>MGRENVLPVHNDVYEDFVFTTPYFQPESTFKSVPKLFSDILLGGVEWVYTTSESVLAYDYKLWYLWSGVSNLDESFDMFFNQYWALSLSTSVFQLFYAVILDRYLSVLFQNTPYTNDWFRMMLHSKETALIWLYHPELSWHINGLNQFFTYFYGGILEFVYFDKSNPDMCILVHTLWIHLLILFLIFTGFVTILFSFYGNPNTEENTIDSDYLAASGTVEAEKEITSIDDYLGLVFAIAYVFGVFFYVHGWTSMLSHAVLLLSCYSIIIMFLFILGMPTLLLYDFGIFFLAYLKGAGKYISSVAEMMFDYTACLVFYIRILAQWIRVVLMVVTFISLSHYVSDFDITNSALIGSENQSDSMNELNTNFSMTYYILTVLPGKFIYWIYEILHTFFVVCSQFVAFFAIVFWLFLFLYTFFIIEKHEDFFSKKREERKKKLKELWNLKN[2x];>MIRNFHSLVKRVPRLALTPFFGFRTSMTLADKKLSTGEASVVLAEKIKGITQQNDITEYGTVISIGDGIARVFGLTKVQAGEMVEFKSGIRGMALNLETDNVGVVVLGNDRDIKEGDVVKRTGAIVDVPIGEAMCGRVFDALGNPIDGLGPLKTTQRARVEIKAPGIIPRQSVRQPMQTGIKCVDSLVPIGRGQRELIIGDRQTGKTAIAIDTILNQKEAFNTGDVKKQLYCIYVAVGQKRSTIANLVSILKQHDCMKFTIVVCATASDAAPLQFLAPYSGCAIGEFFRDNGKHALIIYDDLSKQAVAYRQMSLLLRRPPGREAYPGDVFYLHSRLLERAAKMNDSLGGGSLTALPVIETQAGDVSAYIPTNVISITDGQIFLETELFYKGIRPAINVGLSVSRVGSAAQIKAMKKIAGNLKLTLATYRELAAFSQFGSDLDAKTQQQLNTGERLVEMLKQNQYTPMKVEEQVCIIFAGVKGFLDALVTSEVLKFEKKFLEHVRTNHSALLKRIRDSGDLSEVDTNELNTIIPLFIQEGGFKLKAQ[6x];>[2x]MHSTLRVFTKNNCLSFTNMNRFSTAAQVAQANYSKFRADYSASVAAFQQRIKTIEKENTGSMKKPMAKAYEHPYNSEHHPLNFSAVKIAETFHDFIGPEQVSPHYESFAMSRKFLLTFWGGFFVLNFGMATVDLNWIMKSTYIPWIFWFQLMYFYVEGKNSMFMPLLQRFYRRAAANEIFTMEAFYHENIENKLRNLMRITKGQLEYWDIHTSYGEIRADSINNFLANEYLRLQSHITSRALNILKQAQAYETMNQAALLQKLIDDATSAIDNALKGDKKAEVLARSLDSAIDGLSKGYMDYQNDPLLPLILSSIEANVKKITTLSAQEQANLIGLTAEQLKSIKENDVRARKEFLESQPKLDNNLKNIESVKKILATWGK;>[2x]MITILDYLFLLDLNDDLTRKAVFEQVIIFIFIYCTMNFLAWSTVVELIWPTHFFNRRHSSSQEFIRFRTYTEVLLKISAYNDFFYVLNNYYYNQKLILKN;>[2x]MSMLAKIAKNVVKTQALKNTTAAQTPSFQAPGNQDKILKWISTLSNKATTGESRSYCTQLSSLVSFYNKQHVEQIPTIDFNEWKSVISTQGLVDKVKENYESLIKEQYNTDAISKQISSASSKALDDIENELSFHAAIWLNAYADYTMFLFELEEYNDPNDYLMHENFDFFRGLETELEELTETHNYIPGAKDDVNLRGYLATQFAWGKKVISFYRHPADDFKCAKATKNMLGR;>[6x]MLSKALQRGIARAFSTTAKKEAPKTVKANGQVSQVIGAVVDVQFEGELPQILNALEVQGTQHRLVLEVAQHLGDSRVRTIAMDSTEGLVRGQPVVDTGLPISVPVGPGTLGRIMNVIGEPIDQRGPIKAAKLYPIHRDAPSFTDQATSAEILVTGIKVVDLLAPYARGGKIGLFGGAGVGKTVLIQELINNVAKHHGGYSVFAGVGERTREGNDLYHEMMDSKVISVKEGESRCALIFGQMNEPPGARARVGLTGLTVAEYFRDEEGKDVLLFVDNIFRFTQACSEVSALLGRIPSAVGYQPTLATDLGALQERITTTQKGSITSVQAIYVPADDLTDPAPATTFAHLDATTVLNRGLTELGIYPAVDPLDSTSRMLDPITIGEEHYTVARGVQKLLQDYKSLQDIIAILGVDDLSEEDKLVVARARKVQKFLSQPFFMSEVFSGIPGRFVNLKQNIASFKALLEGAGDEYPESCFYMKGDLEESLAAGRADALKSK;>[2x]MIHCLRNIRTVSALQSKISYNLGGGNKRKKTSGDLDNYDVLFVGANLGGICSNHFDKDTHGKYKCFVSFDQPINQIYSVRIPYEQQRVRKSEYIHFSKKSINQFTPSEMLAVKEILPEQNAVVLSSGRRIGYNQLVLATGLKHDFSQIKGFYEALEHPEHPVYANRDPETWRSAQHKYSKYISNFKSGDGYFCIPEYPYAGEVECFNFFVSDEVWKWAQHHGALSPKHTFTIVNANEKFVHYCDSADAFIKERLEKRGIRVEYNTKLLEVHQDGQKATFINTKTGEKSVRDYNNLYSIVPSKRQEFLDKAGLTNGNGLLNVDHQTLQHKKYKNIFGLGDAADLPTTKTFWAGWYQIAVVRNNVKRNLQGQTLNAHYDGFSKVPLFTGHQTLTYVAHSYGGVGNWQHLKHNNGGILAWMRYRSWAKGMAKKFQDFYNGARLGPPYHKVLKSFPELPGSPESQQSSGISKYFPTKTENKAAH;>MSLHEKMQTDYLWVKDHSQADSWAKARTHGYNYIAHTVPNKKERYEMIWRSMGKSTDWELEKFRLGKKFPDRGNKRRWFKNLFRLIKNPMGYIFWKTYKARLAKPSLIVTSMFIGFTLGFIKLKAQSIAYSKKQYATLRAGKNIEGSGQVHFGYHDQKWGMPAIPMFQLMYYELPGNSIVVNPCRNQNYRLYFEMRKKLGILPA[2x];>[2x]MINRSTAFISKNLRQANLTQSSLAMKTQYNQMGFSSDNPYNKRWEYKWKHSYYTYPRDYEHTEVRKPQDSKDVPPIYFAYYKDFVDRWLPGMNMWWQRRHRIFDKFNVYFLPGMSLFFYQFADLALGFKIMAAFPLFLAYTRIRDKTLDPDFKETYLRDMIYQNPEITKYFNEETIHVLDYEFEYLPGYLCPEKFPEYQNKTWQFFNTDTAQAEGFFKFGDVESGATMTLKFKTMPIPGKFRYQVGEPFYFYDLRAEIKCDGVYKEVVLVDEKESLKKIRPFLFLI;>[2x]MQVIRKHLAQKGLFNPFLFNRFSTQQDITSVPGDKPPAIEDSIHGKYAGVLFSSASSNKSLNKVAEDMKYFNQLYKESEVFKSFLNNVSLKRNQQRDIISALGKTNFNPATNNLLETLIENKRLDSLPKIAEKYMDYYRILNKQESITIISAQELTAAEKQKVEQGLKKGNANVQFTVVYQVDPAILGGLQMYSGNNFLDCSLLSRVNKLKTEIAKISF;>MQQRKKIYLRQKRKIYIQLKNKEKKKNNQFIQKREKMGYKIRNKSIFWTRAGWKNNWHPKNFNAPRPSYGEFTMGIRCRNDHHSFLRYVQTYRNMSRHCKQYFLGDKQLEETFILGLRSLFLVPYDSQCLTDQIKHGGERRFVDQLDRDFELISYNTHPYQLFTYTVRNEHLAWKNEQYEKIQKGEKTFEQELLDYLDEQVLAEKAKLRDGQNFSIERMTEIALHVFRKARAGKVRPAQDVRGPDGNVNDFLEQRRPFEHPNPTGVTH[2x];>[20x]MLLVKAVKVLVMGGCMLPIAFGALGTGVLFAGFNVALSRNPEETESLFNNTLMGFALIETFIFMSIGLGFFVLFAA;>MNPIQKAWLKILEPVSYVINEKMAKRTGIIGKLGRFFAIGPREYGVHPINRMFIFMNRKYMAFQAVALHRYSFVKSLTHNGFHMLRVFRHFAFVLPATVLAGLGLFVYWGDDNKCYSPDRFPYLKKRAGDMALPLNSLNQRTSAHYIEINAIYGAEMMKRYHKVWENIIEERSKATDQEKKTRYAHPSYQYSPLPVVSIPNVLNPLNLQ[2x];>[2x]MSENKAPGQIYAYDIHNTHYPYVNIKQDSQTQLLASFRRSIASINPFSYRQVPSQDRAAFGLRWGNAWYAPNPYPNGIHFDRVFPTHYDPLAETNRTKANLQLIKYAPGNYSTLVVTSEKLPRPCIRTIQNYRRCQMVNGTEKCNSEAQDILAICPNWALDHMKEKVRFYTKALAINNQTYIRAMQVEEYNQGRTVADVAPKTWIHGTRQHLRPDTMWADDRYTNITQTEINEAIKRVEARKAREHEKKPVEQANVNANTGEQPVRVEKSLYP;>[2x]MWYKYFSKQSWNLRVWRKANLKYNQDDFGMTQPKYIARFGDFRFRLVRTEGALRGCMFFVGFGCFSIINYLYGRYGYIINESSQKRAAQDLLDNDMAADKILFKNRVGAPTRPLRSLDDMMAFLSGSATYDQLADYASYNHAMDVNQDQQAGLDSWMSEKDKNMVKYYQRSLGKKVEGI;>[2x]MPVKEGQAKLWFSTKEEADAYDDKMISNIELKSQDYEDENFSPVFNRKTQEYFLEPSEKFKSDFAELLRPLRSLSFNQVVDRYVLIPPNHTFYRNWTYEKFLGGFGLSYLILRELPLRNFYARVFVMYAFAAKVLDHLGNPFPFSGHGQIVAAADRWNHWDVRCYDNVMKALKYIRIPTVQNNIPEATRWYGRQPGHLLRADTYWIPNLVSQRFAKHQPAHWDGTQNMPIFRLADPKHKDSYMVQFR;>[2x]MDNYFTAITLLGLRDQNLPPFKDARLQRYKSIKKMIDLIETTTKLAPPMPVELFMLNPTDPEWDDDMTYPTITHATALYKSSALAGNLFLYAYNYNNFTANIRLRTMRYLFPVVSLAIFGNIYWDYRSQLVKVNLFDEYIQARAQELVKQNEYLLEHEDVKRYVWWYEDLKETLARVHRQANNHKACDFKDSEIILQDFIRRYTNPKDNLPIKFHPQGQTF;>[2x]MEGFIQNKRKKEKEGEEEEESKEKRKQINQLNKQKQEEEKIYQQKKDQKRKKYLYQRKEMTIFAETWEASEYQYRNKANLKTLPVNHLGKLAELKFDFVEYKAHQLIACHLYERMTIHCMNQYGLFKDFYRPECLDAQYYFKTCVELNAAYGIQKKFFPEHFVGSPYARPVPQFQQLGL;>[2x]MKQKINKLLKNKGVQDKYKYLSKLILLDQEIKGKIKRKNKKEKQKRKNKLILEEMQNTTNIVHVPVHMGHTHYFDYIDSFPKLKEGPTLEENHITNQKILREQLISGQQGLEQNLCLRNCFKLSQKRYIEFCLDRKCGGADFQRAATILGYTKN;>MSNIFLELQDGDKTVYTHTSLIEESKQEQIQAIYDKVPQWTNGGRFLGFWLSMEAVNRVQSVAKLPIYYRAGIVATSTLLGGLVSSLVFWKSGNENQVAKLANGAPVYLKKWEVPELSKLYFFLDDDNNFKPSLNHHAVTQGRQYYKIYQHN[2x];>MFRNILSLVTKPSKLSQKTFYNFAAAKNEVQVSKKQQQAGAKRDLTQYVEGQIVNRNQLTLKKQEDIEQYVLKLVRGYFRTTNKQGLNINSVLQDHGLDEFDSIELAMQVEEDLGYVISAETIPVLNKVKHFVNYINHVEQFKAENGKAPIA[2x];>[2x]MSQDPKIVNPQLWPNPNKLRFADLYKYQGVEMKKINDSIKNYKAAKFYIGGILGGCLVFKFFIDAAVDKYIFGENGNGGKFLEMQTINSNYDYYYNRQFQRMRYLTEDPAGDDPLQKTKDEHLVDLGFIPKVFGANVEVRKRAPHDKYL;>MNSLSSKKANSLVFKSIRNFTLQWGSLAERPMVDRVMSTSTWPVPYYQRLFKAYPIREKKDKMSLLLSDIDIDDTNWYQAKDFLRGSFRGRQIVDYVENNIASNTYILIQQDVANMAKAYVHDICGYIDVANKENVRILSKGDLI[2x];>[2x]MFTRFVTQPTLLTQTQRALFSALTKKQKMEVTLRTPYKEYLANFDGFSRITAKTNEASLVIQNKTPASLYVLPPGPLKIRFTSEVKNVSGDFLHTGGWVIVHADNTCEINVMDLFDRKEVRADQFEKGNIQDLDTLAGKYAAKSRKSTVRLFTKATTQ;>[2x]MCIEFAFKKAGIPIVRNFLHSTEGVIYGLPQRVQRNLAINYTVKQYKEGKAVSAKTIKTLQEAFPSKGDTK;>[2x]MFGLASKGFINTSLVMVPQMNFGANLKQLKIRMKAIGSIKKITKAMKMVAASKMKAETSRLENGRNFAVGSVQKMLENESYVQKKKSTTAPKSTLLVPITSDKGLCGSVNSSIVREVKRLALNNRSAFGLLPVGEKGSSGLSRPFPDLLKSSIVNIQNVNFPTAAAIAHQVSTQGAGYDQVTLIYNHFKNAISYVVKHQELLPRAQFLNLFKYVTRHEAVEPELEYSKNYFFELYMASSVYNALLNSSASEQASRMNAMENASKNAGEILSKLTLDYNKARQAKITMELIEIISGASIV;>MNRSVNIAKNLIQTYRAMSVQSRFAFSTREEEWLDKRTKSQEKVYFDQEDRKAMKRLLEKLNTTSKFVEDSEYLAPQNLEVENILKRYHINYTQALIDELVDWKTGKN[2x];> MKMEYLQSEEKKDAINKQIHKKEEKEEKEIKIKRKNKVKQRIQIINQIKKYIEAKQQKKQIQSKNQRKYKGRMINTRKQVFKCLWGAQPAYNFSRIINHLRGDPVYQDNTKDVSLRGTFLRGKYDDLPTMIFFTEACDLTANWIPFFTNPQYDILAHRNVWLLNPRNFGNSDRHPSFDLQEMSDDVMRFMYSQKISMATLGGHGIGGKIALAVGCYHAERVTGVFSIDSSPMDQRYHEAFKEFKGYVNALTEINFKTWSDKDVKVFLKENIKDPKWRSIFTNNISKNAKTQSDSFNFEINYLNHNLNFNKADSLGNWAVKNGIYTGRAHFIFPEYSRWVHLATNTLPMHKVCARVKGFGHDIFYVQGDENPLNHWVYDFENYANVVASKLNKFLHSYDGVHALLKDRTEIGNFMIPDRIKSRNDSKHIYGDYSPAHLHHNWRFNHIYEKHDELDKKLNEQ

The F-type ATP synthase (F1Fo-ATP synthase) is responsible for generating most of the cellular adenosine triphosphate (ATP) from adenosine diphosphate (ADP) and inorganic phosphate through rotary catalysis. In eukaryotes, ATP synthases are found in the inner mitochondrial membrane. The type III ATP synthase was detected in ciliates where it induces tubulation of the cristae membranes. In this study, we present the cryo-EM structures of the type III ATP synthase dimer and tetramer with associated lipids from the model organism Tetrahymena thermophila in complex with the natural inhibitor IF1.

Refinement into a 2.7-Å resolution allowed for construction of a of the ATP synthase dimer. The overall structure of the type III ATP synthase dimer has a U-shape, with no other types detected, which is consistent with previous low-resolution studies. The ~2 MDa complex comprises 81 protein subunits, 9 of which were not previously reported, and assigned directly from our cryo-EM density map. The overall size of the type III ATP synthase dimer is substantially larger than its counterparts. The specific subunits at the altered interacting surface stably tie the two monomers together in parallel to each other, with little induction of membrane curvature. The total surface area buried between the monomers exceeds 16,000 Å2, which is at least four times more than for the characterized other types. Homotypic subunit-b contacts also involve bound cardiolipins, whereas subunit-f interface involves  protein contacts only. Consequently, the type III ATP synthase dimer structure contains by far the most extensive dimer interface observed in any reported ATP synthase dimer. Two copies of the ATP synthase dimer model were refined into the Fo-tetramer map generating a composite ATP synthase tetramer model. Both monomers are inhibited in the same rotary state by the natural inhibitor IF1. In addition, ATPTT2 has evolved a unique function as a platform for the binding of the natural inhibitor IF1 in a way that inhibits both monomers in the dimer, which was not observed before.ARABINOSE-5-PHOSPHATE | C5 H13 O8 P 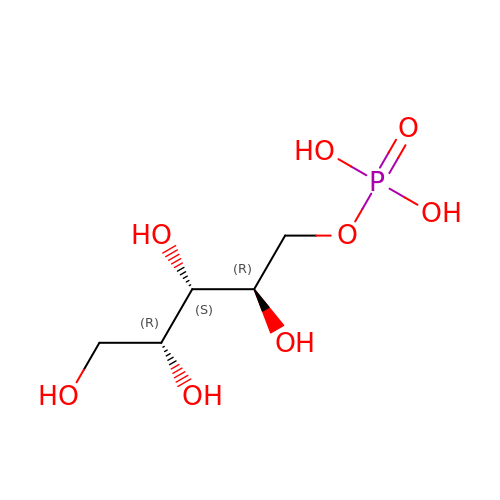| VJDOAZKNBQCAGE-WDCZJNDASA-N> MKHHHHHHMKQNSPLDEENLTQENQDRGTHVDRGLASANVDFAFSLYKQLVLKAPDKNVIFSPLSISTALAFLSLGAHNTTLTEILKGLKFNLTETSEAEIHQSFQHLLRTLNQSSDELQLSMGNAMFVKEQLSLLDRFTEDAKRLYGSEAFATDFQDSAAAKKLINDYVKNGTRGKITDLIKDLDSQTMMVLVNYIFFKAKFEMPFDPQDTHQSRFYLSKKKYVMVPMMSLHHLTIPYFRDEELSCTVVQLNYTGNASALFILPDQDKMEEVEAMLSQETLSRFFDSLEFREIGELYLPKFSISRDYNLNDILLQLGIEEAFTSKAD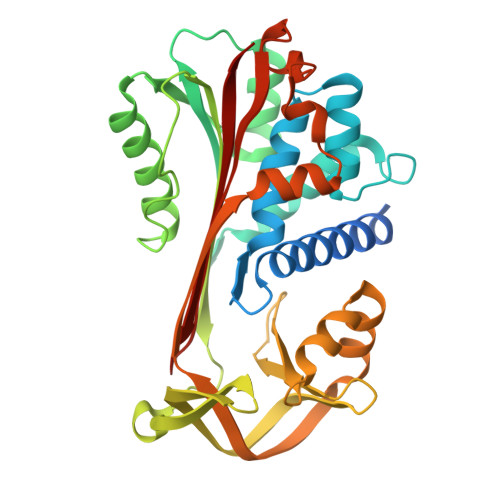LSGITGARNLAVSQVVHKAVLDVFEEGTERSAATALEVLFQ>MRSRRVDVMDVMNRLILAMDLMNRDDALRVTGEVREYIDTVKIGYPLVLSEGMDIIAEFRKRFGCRIIADFKVADIPETNEKICRATFKAGADAIIVHGFPGADSVRACLNVAEEMGREVFLLTEMSHPGAEMFIQGAADEIARMGVDLGVKNYVGPSTRPERLSRLREIIGQDSFLISPGVGAQGGDPGETLRFADAIIVGRSIYLADNPAAAAAGIIESIKDLLNP[13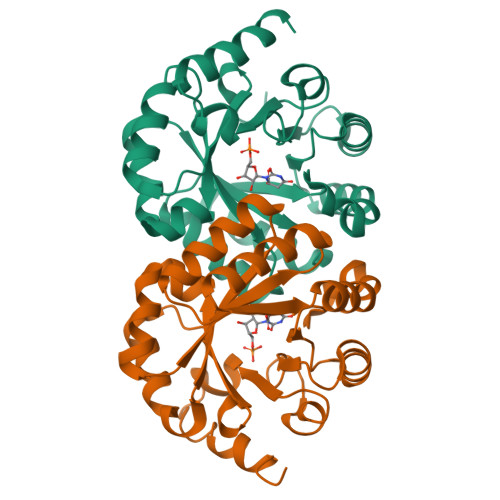x]>SMEHATPCIKAISPSEGWTTGGATVIIIGDNFFDGLQVIFGTMLVWSELITPHAIRVQTPPRHIPGVVEVTLSYKSKQFCKGTPGRFIYTALN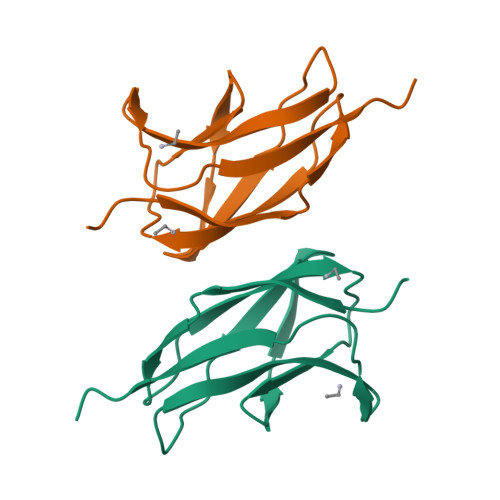EPT[3x]>MTDTPFIRPDMKAFLEAIAAMAGPTLAEMTLEEARASYVALHGMADRPARELAVIRNLSCPGPAGDIPLRLYDARESREAGPVITFYHGGGFVIGDLDTHHNLCTEIAALMDLPVVAVDYRLAPEHPFPAAIEDCEAATRWVASSPSELGRTASGVIPIGDSAGGNATIVVSQLLGAKPADVPVVLQVPIFPLASDAVGSASLEAFAEGFVLTKASIEFFDTAYKADRADPRGFPILGDHTAAPPTIVATASLDPIRDSGRDYAKALVEAGRDVVYLEMEGVTHGFTNIRAAVPSTQGDLERIIAAMKMMLGTA[4x]

To advance the understanding of esterases, we have identified and characterized E53, an alkalophilic esterase from a marine bacterium Erythrobacter longus. Family IV esterases, to which E53 belongs, are widely distributed in microorganisms, plants, and animals, specifically degrade short-chain esters. The family IV esterase can be characterized by the α/β-fold hydrolase group, and contains two distinct structural domains: an N-terminal CAP domain and a C-terminal catalytic domain. The catalytic reaction relies on the S-H-D/E catalytic triad located in the catalytic domain.

The conserved tyrosine was replaced by phenylalanine at position 191, while the conserved glycine was replaced by serine at position 285 in E53. In our work, F191 and S285 in E53 were mutated to the conserved amino acids, and D161 and N288 were replaced with alanine. The variants, D161A, S285G, and N288A, did not change the specificity but dramatically reduced the enzymatic activity (> 90% loss of function) on p-NP ester hydrolysis, demonstrating their crucial roles in the catalytic reaction. The unexpected outcome was S285G: most esterases have glycine at position 285; after mutating the serine to the more conserved glycine, only 20–30% of activity was detected. From the structure, the shortest distance from S285 to the bound substrate is 3.0 Å, suggesting S285 could be involved in the coordination of the substrate. Substituting this serine with glycine could impede this interaction, leading to the decrease of the activity. Despite the fact that S285 is adjacent to H284, a residue of the catalytic triad, the crystal structure of E53-S285G did not exhibit obvious relocation of the catalytic triad (2.7Å for H284Nε2 to S162Oγ, and 2.6Å for H284Nδ1 to D254Oδ2) compared with WT E53 (2.9 Å for H284Nε2 to S162Oγ, and 2.6Å for H284Nδ1 to D254Oδ2). The distance between S162Oγ to the carbonyl carbon of ester bond was 4.6 Å in WT E53, 4.6 Å in E53-I256L, and 4.0 Å in E53-S285G. Such distance could allow the catalytic process to happen.4-fluoro-N'-[(3-hydroxyphenyl)sulfonyl]-5-methyl[1,1'-biphenyl]-3-carbohydrazide | C20 H17 F N2 O4 S 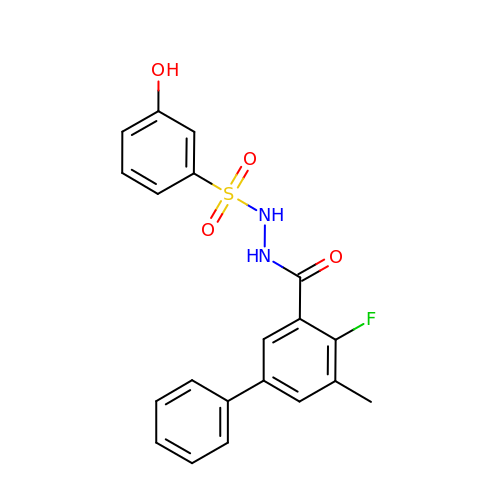| KVJFJJXCBRSCDY-UHFFFAOYSA-N4-{[(2-amino-4-oxo-3,4,7,8-tetrahydropteridin-6-yl)methyl]amino}-N-(1,3-thiazol-2-yl)benzenesulfonamide | C16 H16 N8 O3 S2 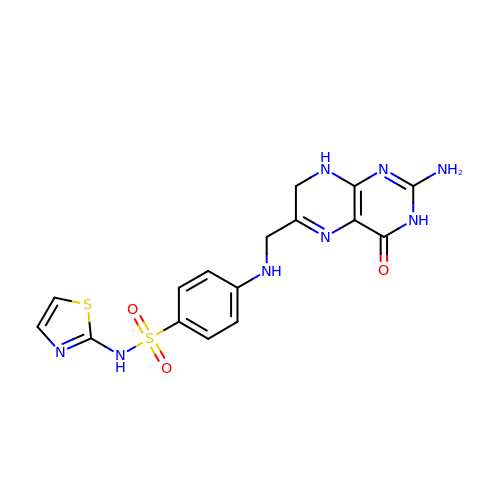| XKJZNFKQXDBJHJ-UHFFFAOYSA-N>VHHPPSYVAHLASDFGVRVFQQVAQASKDRNVVFSPYGVASVLAMLQLTTGGETQQQIQAAMGFKIDDKGMAPALRHLYKELMGPWNKDEISTTDAIFVQRDLKLVQGFMPHFFRLFRSTVKQVDFSEVERARFIINDWVKTHTKGMISHLLGTGAVQQLTRLVLVNALYFNGQWKTPFPDSSTHRRLFHKSDGSTVSVPMMAQTNKFNYTEFTTPDGHYYDILELPYHGDTLSMFIAAPYEKEVPLSALTNILSAQLISHWKGNMTRLPRLLVLPKFSLETEVDLRKPLENLGMTDMFRQFQADFTSLSDQEPLHVALALQK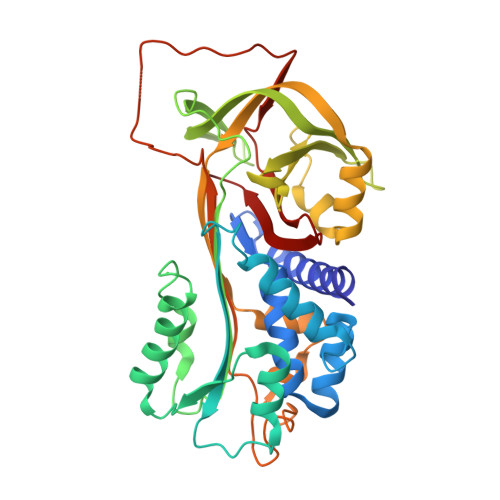VKIEVNESGTVASSSTAVIVSARMAPEEIIIDRPFLFVVRHNPTGTVLFMGQVMEP[4x]Presequence protease (PreP), a 117 kDa mitochondrial M16C metalloprotease vital for mitochondrial proteostasis, degrades presequence peptides cleaved off from nuclear-encoded proteins and other aggregation-prone peptides, such as amyloid β (Aβ). Of the Aβ-degrading proteases, PreP belongs to the chamber-containing protease (crypt-containing peptidase, or cryptidase) family that uses a sizable catalytic chamber to engulf, unfold, and degrade their substrates. PreP-N and PreP-C, in the closed state of PreP, form an enclosed catalytic chamber to entrap and degrade monomeric amyloidogenic peptides, thereby preventing the formation of toxic aggregates. Comparison of the five cryoEM structures derived from the apo- and substrate-bound PreP reveals three key conformational states based on the degree of opening of the catalytic chamber: open (O), partially open (either pO1 or pO2), and partially closed (pC).

3D classification of PreP particles revealed three distinct open state structures of PreP. They were refined to an open state (O) and two partially open states (pO1 and pO2) with resolutions of 4, 3.7, 3.9, respectively. Apo-PreP has three states, O, pO1, and pO2 that are distinct from each other with the two pO states being slightly more open than the pC or C states. Of these structures, the pO, pC, and C states of PreP have a small variation in the degree of opening, making their chamber inaccessible to substrate binding. 3D classification revealed that most PreP particles (~74%) were in the partially open (pO) states, indicating that PreP in the absence of substrate prefers to be in a state inaccessible to substrate binding. Consistent with the cryoEM data, the SEC-SAXS data confirms that apo-PreP in solution also prefers to adopt the pO state (72% based on OLIGOMER and 90% based on ensemble optimization modeling (EOM)). The fact that PreP in solution prefers the pO state rather than the open state is logical because the transition from the pO states to O state loses substantial buried surface (650–940 Å2) and a network of hydrogen bonds and salt bridges, and thus is energetically unfavorable. The switch A and C regions in the pO states have lower resolution and higher thermal B factors than the rest of PreP structures. As switch A contains residues involved in substrate peptide binding and catalytic zinc ion coordination, such high dynamics would render the pO state catalytically incompetent. The transition from the pO states to O states allows the capture of the substrate, and thus is a key state in the catalytic cycle.

> MHHHHHHAAACERALQYKLGDKIHGFTVNQVTSVPELFLTAVKLTHDDTGARYLHLAREDTNNLFSVQFRTTPMDSTGVPHILEHTVLCGSQKYPCRDPFFKMLNRSLSTFMNAFTASDYTLYPFSTQNPKDFQNLLSVYLDATFFPCLRELDFWQEGWRLEHENPSDPQTPLVFKGVVFNEMKGAFTDNERIFSQHLQNRLLPDHTYSVVSGGDPLCIPELTWEQLKQFHATHYHPSNARFFTYGNFPLEQHLKQIHEEALSKFQKIEPSTVVPAQTPWDKPREFQITCGPDSFATDPSKQTTVSVSFLLPDITDTFEAFTLSLLSSLLTSGPNSPFYKALIESGLGTDFSPDVGYNGYTREAYFSVGLQGIVEKDIETVRSLIDRTIDEVVEKGFEDDRIEALLHKIEIQMKHQSTSFGLMLTSYIASCWNHDGDPVELLKLGNQLAKFRQCLQENPKFLQEKVKQYFKNNQHKLTLSMRPDDKYHEKQAQVEATKLKQKVEALSPGDRQQIYEKGLELRSQQSKPQDASCLPALKVSDIEPTIPVTELDVVLTAGDIPVQYCAQPTNGMVYFRAFSSLNTLPEELRPYVPLFCSVLTKLGCGLLDYREQAQQIELKTGGMSASPHVLPDDSHMDTYEQGVLFSSLCLDRNLPDMMQLWSEIFNNPCFEEEEHFKVLVKMTAQELANGIPDSGHLYASIRAGRTLTPAGDLQETFSGMDQVRLMKRIAEMTDIKPILRKLPRIKKHLLNGDNMRCSVNATPQQMPQTEKAVEDFLRSIGRSKKERRPVRPHTVEKPVPSSSGGDAHVPHGSQVIRKLVMEPTFKPWQMKTHFLMPFPVNYVGECIRTVPYTDPDHASLKILARLMTAKFLHTEIREKGGAYGGGAKLSHNGIFTLYSYRDPNTIETLQSFGKAVDWAKSGKFTQQDIDEAKLSVFSTVDAPVAPSDKGMDHFLYGLSDEMKQAHREQLFAVSHDKLLAVSDRYLGTGKSTHGLAILGPENPKIAKDPSWIIR>[2x]AAAEIETIVRESEANRIQAQTWFSHPEKSKVSFRYDERETSSIRSISIETFLSFYSSKFNREPYSVLDIGCGQGQVIQYLNSRFQKIELTGIDSSAQAISSAKKLGINASFICSNAENIMQYVSKKQDIIFIHLCFGLFKNPIAIVNTLIHLLSDQSCIYIVDLDRNSLGEG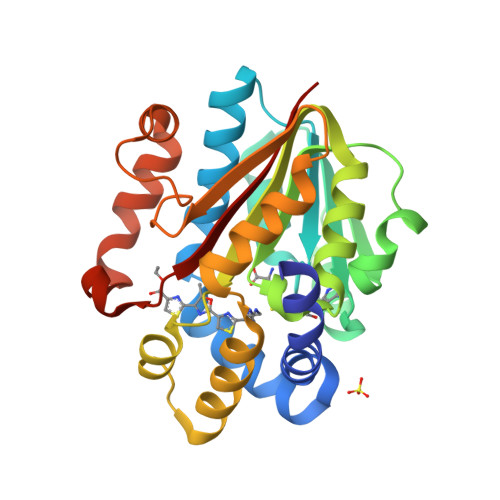LNTAQSREEEAYLKDQYRASLTMEEFKQLLHVVTKEQHGVSFHVGNSFIGGFDETSSQFFSLMRNRNLQDALRTSVGEQLKQSQMPALLHGWIIKNKRYT>[2x]MHHHHHHENLYFQGMRVAMMTREYPPEVYGGAGVHVTELVAQLRKLCDVDVHCMGAPRDGAYVAHPDPTLRGANAALTMLSADLNMVNNAEAATVVHSHTWYTGLAGHLASLLYGVPHVLTAHSLEPLRPWKAEQLGGGYQVSSWVERTAVEAADAVIAVSSGMRDDVLRTYPALDPDRVHVVRNGIDTTVWYPAEPGPDESVLAELGVDLNRPIVAFVGRITRQKGVAHLVAAAHRFAPDVQLVLCAGAPDTPQIAEEVSSAVQQLAQARTGVFWVREMLPTHKIREILSAATVFVCPSVYEPLGIVNLEAMACATAVVASDVGGIPEVVADGRTGLLVHYDANDTEAYEARLAEAVNSLVADPDRAREYGVAGRERCIEEFSWAHIAEQTLEIYRKVSA

Mycobacterium tuberculosis produces glycogen (also known as α-glucan) to help evade human immunity. This pathogen uses the GlgE pathway to generate glycogen rather than the more well known glycogen synthase GlgA pathway, which is absent in this bacterium. One of the routes to α-maltose-1-phosphate is now known to involve the GlgA homologue GlgM, which uses ADP-glucose as a donor and α-glucose-1-phosphate as an acceptor. Thus, the enzyme uses ADP-glucose as the donor and α-glucose-1-phosphate as the acceptor.

Attempts to crystallize the α-maltose-1-phosphate synthase GlgM from M. tuberculosis were unsuccessful. We therefore switched our focus to the GlgM homologue from M. smegmatis, which shares 77% identity with the enzyme from M. tuberculosis. To help compare GlgA (a GT5 family member) with GlgM enzymes (GT4 family members), the X-ray crystal structure of GlgM from Mycobacterium smegmatis was solved to 1.9 Å resolution. The structural similarity between these proteins confirmed that GlgM had a GT-B fold. While the enzymes shared a GT-B fold and several residues responsible for binding the donor substrate, they differed in some secondary-structural details, particularly in the N-terminal domain, which would be expected to be largely responsible for their different acceptor-substrate specificities. Confirmation that GlgM forms a dimer in solution was obtained using size-exclusion chromatography. This indicated a molecular mass of 107 kDa, which is close to the theoretical mass of a dimer (87 kDa); the slight overestimation of this value could be owing to the elongated aspect of the GlgM homodimer. The kinetics of the enzyme conformed to a ternary-complex mechanism. Although the M. tuberculosis GlgM enzyme exhibited a trace of glycogen synthase activity, which was three orders of magnitude lower than its α-maltose-1-phosphate synthase activity, the M. smegmatis enzyme exhibited no detectable glycogen synthase activity. Likewise, we have been unable to date to obtain ligand-bound structures of GlgM, making it difficult to rationalize these structural differences with respect to function.>MELRHIRYFLAVAEERHFTRAAARLGIGQPPLSQQIKDLERELGALLFRRVSYGAELTEAGIAFLDVVKEIPVMAERATQAAQRAVRGELGVLRVGFTASSAFNSVVPTAIRAFRRAYPDVRLQLEEDNTTRLADGLNEGSLDVAFLRPGFAGSERFHLRMLSEEPMMIVMAENHPAASYEEISLSAFRDETFLLFPREIGLTLYDSVIESCRTAGFEPTIGQLAPQIASVINLVAAEMGVSIVPASMSQVKVIGVVYRHIADQTPTAKLALAYRRGDTSPVLRNFVLTVFP[8x]

The bacterial protein ItcR is unique in its ability to bind to itaconate. Structurally, ItcR is a transcriptional regulator protein with an N-terminal DNA-binding helix-turn-helix motif and a C-terminal itaconate-binding domain (IBD)24. Multiangle light scattering (MALS) analysis showed that IBD appears as homodimer in solution. Here, we report the development of a highly responsive, genetically encoded itaconate fluorescent biosensor, referred to as BioITA (biosensor for itaconate).

Furthermore, the crystal structure of IBD without or with itaconate binding was determined by multiple-wavelength anomalous diffraction and refined at a resolution of 3.25 and 1.48 Å, respectively. In line with the result of MALS, the IBD proteins form a homodimer in both of the apo and itaconate bound states. Notably, alignment between the structures of IBD in the apo and itaconate bound states demonstrated that monomer in each dimer exhibited translocation of over 7 and 10 Å in the N- and C-termini, respectively.> MAHHHHHHMKTGDTVADFELPDQTGTPRRLSVLLSDGPVVLFFYPAAMTPGCTKEACHFRDLAKEFAEVRASRVGISTDPVRKQAKFAEVRRFDYPLLSDAQGTVAAQFGVKRGLLGKLMPVKRTTFVIDTDRKVLDVISSEFSMDAHADKALATLRAIR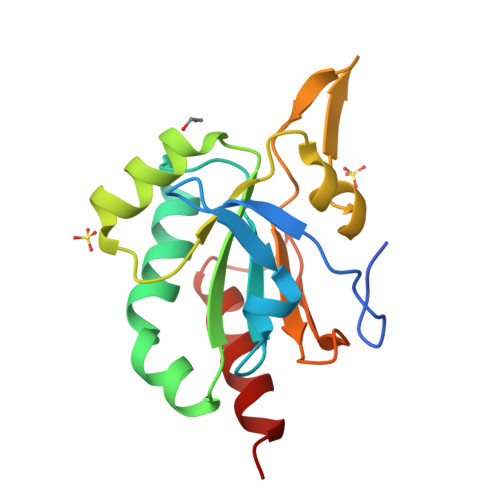SG> PISPIETVPVKLKPGMDGPKVKQWPLTEEKIKALVEICTEMEKEGKISKIGPENPYNTPVFAIKKKDSTKWRKLVDFRELNKRTQDFWEVQLGIPHPAGLKKKKSVTVLDVGDAYFSVPLDEDFRKYTAFTIPSINNETPGIRYQYNVLPQGWKGSPAIFQSSMTKILEPFKKQNPDIVIYQYMDDLYVGSDLEIGQHRTKIEELRQHLLRWGLTTPDKKHQKEPPFLWMGYELHPDKWTVQPIVLPEKDSWTVNDIQKLVGKLNWASQIYPGIKVRQLSKLLRGTKALTEVIPLTEEAELELAENREILKEPVHGVYYDPSKDLIAEIQKQGQGQWTYQIYQEPFKNLKTGKYARMRGAHTNDVKQLTEAVQKITTESIVIWGKTPKFKLPIQKETWETWWTEYWQATWIPEWEFVNTPPLV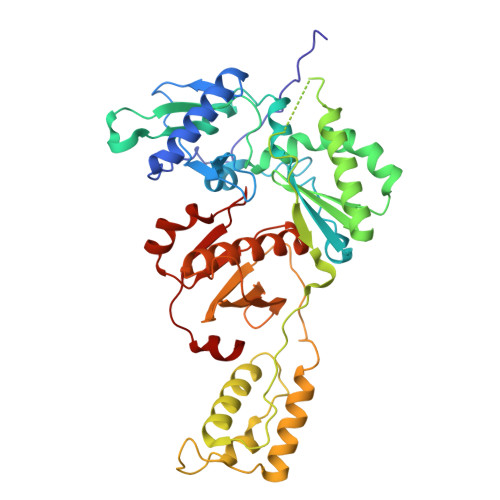KLWY> GPGHMVVKFSYMWTINNFSFCREEMGEVIKSSTFSSGANDKLKWCLRVNPKGLDEESKDYLSLYLLLVSCPKSEVRAKFKFSILNAKGEETKAMESQRAYRFVQGKDWGFKK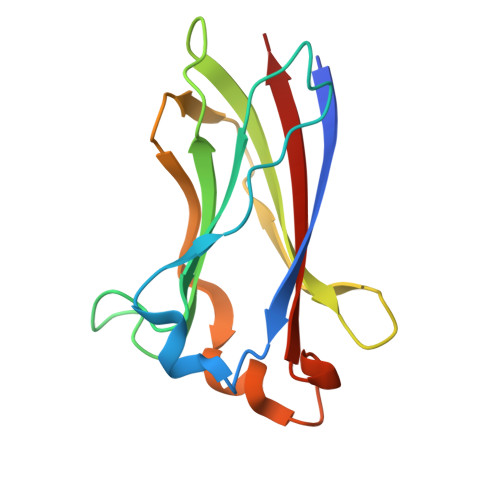FIRRGFLLDEANGLLPDDKLTLFCEVSVVQD>[2x]SGADTGAGAGMFRALFRQAVEDDRYGEFLDVLAEASAFRPQFASPEACSERLDPVLLAGGPTDRAEGRAVLVGCTGTAANGGPHEFLRLSTSFQEERDFLAVPLPGYGTGTGTGTALLPADLDTALDAQARAILRAAGDAPVVLLGHSGGALLAHELAFRLERAHGAPPAGIVLVDPYPPGHQEPIEVWSR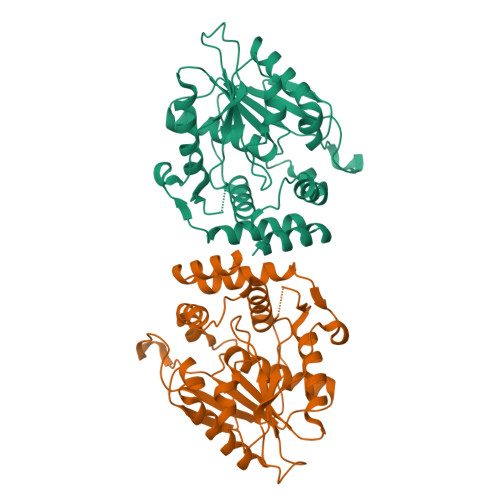QLGEGLFAGELEPMSDARLLAMGRYARFLAGPRPGRSSAPVLLVRASEPLGDWQEERGDWRAHWDLPHTVADVPGDHFTMMRDHAPAVAEAVLSWLDAIEGIEGAGK>VPTLQRDVAIVGAGISGLAAATALRKAGLSVAVIEARDRVGGRTWTDTIDGAVLEIGGQWVSPDQTALISLLDELGLKTFERYREGESVYISSAGERTRYTGDSFPTNETTKKEMDRLIDEMDDLAAQIGAEEPWAHPLARDLDTVSFKQWLINQSDDAEARDNIGLFIAGGMLTKPAHSFSALQAVLMAASAGSFSHLVDEDF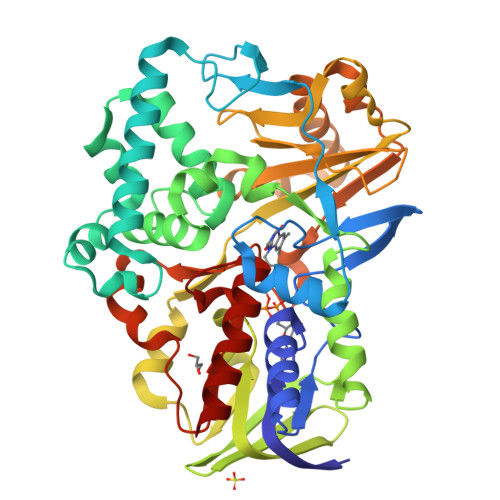ILDKRVIGGMQQVSIRMAEALGDDVFLNAPVRTVKWNESGATVLADGDIRVEASRVILAVPPNLYSRISYDPPLPRRQHQMHQHQSLGLVIKVHAVYETPFWREDGLSGTGFGASEVVQEVYDNTNHEDDRGTLVAFVSDEKADAMFELSAEERKATILASLARYLGPKAEEPVVYYESDWGSEEWTRGCYAASFDLGGLHRYGADSRTPVGPIHFSCSDIAAEGYQHVDGAVRMGQRTAADIIARSKA[2x]> GSMSLNDFLSSVLPVSEQFEYLSLQSIPLETHAVVTPNKDDKRVPKSTIKTQHFFSLFHQGKVFFSLEVYVYVTLWDEADAERLIFVSKADTNGYCNTRVSVRDITKIILEFILSIDPNYYLQKVKPAIRSTC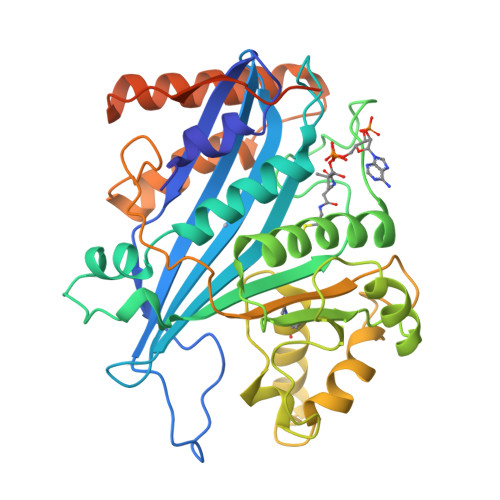PREILTKICLFTRPASQYLFPDSSKNSKKHILNGEELMKWWGFILDRLLIECFQNDTQAKLRIPGEDPARVRSYLRGMKYPLWQVGDIFTSKENSLAVYNIPLFPDDPKARFIHQLAEEDRLLKVSLSSFWIELQERQEFKLSVTSSVMGISGYSLATPSLFPSSADVIVPKSRKQFRAIKKYITGEEYDTEEGAIEAFTNIRDFLLLRMATNLQSLTGKREHRERNQPVPASNINTLAITMLKPRKKAKALPKT4-(furan-2-yl)benzoic acid | C11 H8 O3 | 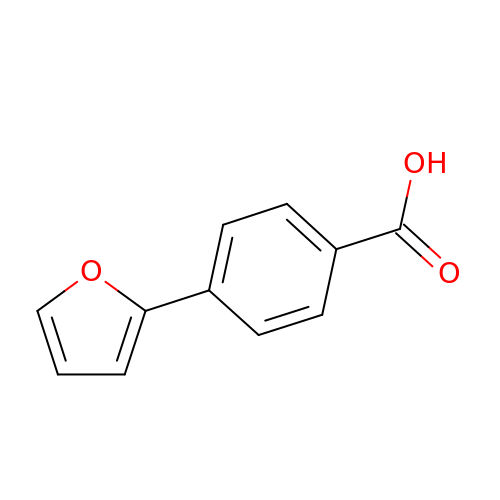FOJYVBSPOBUCMV-UHFFFAOYSA-N>MGRIKNKQFAVIGLGRFGGSIVKELHRMGHEVLAVDIN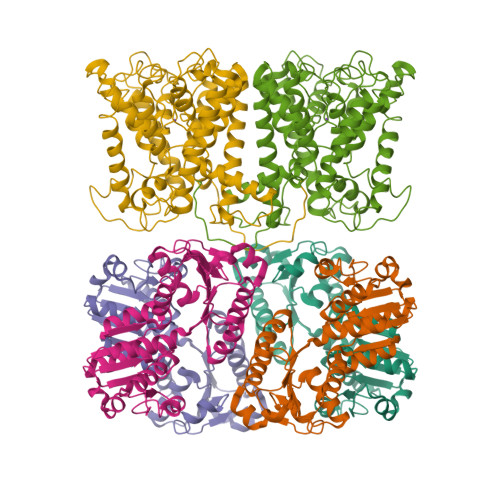EEKVNAYASYATHAVIANATEENELLSLGIRNFEYVIVAIGANIQASTLTTLLLKELDIPNIWVKAQNYYHHKVLEKIGADRIIHPEKDMGVKIAQSLSDENVLNYLEGSKQFAVIGLGRFGGSIVKELHRMGHEVLAVDINEEKVNAYASYATHAVIANATEENELLSLGIRNFEYVIVAIGANIQASTLTTLLLKELDIPNIWVKAQNYYHHKVLEKIGADRIIHPEKDMGVKIAQSLSDENLELVPR[4x];>[4x]MTLQKDKVIKWVRFTPPQVLAIGFFLTIIIGAVLLMLPISTTKPLSWIDALFTAASATTVTGLAVVDTGTQFTVFGQTVIMGLIQIGGLGFMTFAVLIVMILAAAIGLKERMLVQEALNQPTIGGVIGLVKVLFLFSISIELIAALILSIRLVPQYGWSSGLFASLFHAISAFNNAGFSLWPDNLMSYVGDPTVNLVITFLFITGGIGFTVLFDVMKQRRFKTFSLHTALMLTGTLMLNAIAMLTVFILEYSNPGTLGHLAAVDKLWASYFQAVTPRTAGFNSLDFGSMREGTIVFTLLLMFIGAGSASTASGIKLTTFIVILTSVIAYLRGKKETVIFRRSIKYPIIIKALAVSVTSLFIVFLGIFALTITEQAPFLQIVFETFSAFGTVGLTMGLTPELTTAGKCIIIVIMFIGRIGPLTFVFSFAATEQSNIRYPDGEVFTG> GSGAEDGQVEEEPLNSEDDVSDEEGQELFDTENVV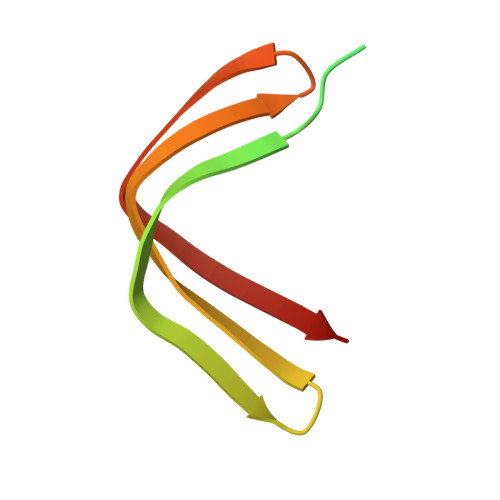VCQYDKIHRSKNKWKFHLKDGIMNLNGRDYIFSKAIGDAEW>GSMSVQSGSTANLPADLATALATAKENDGHDFEAPKVGEDQGSPEVTDGPKTEEELLALEKEKPAEEKPKEDKPAAAKPETPKTVTPEWQTVEKKEQQGTVTIREEKGVRYNQLSSTAQNDNAGKPALFEKKGLTVDANGNATVDLTFKDDSEKGKSRFGVFLKFKDTKNNVFVGYDKDGWFWEYKSPTTSTWYRGSRVAAPETGSTNRLSITLKSDGQLNASNNDVNLFDTVTLP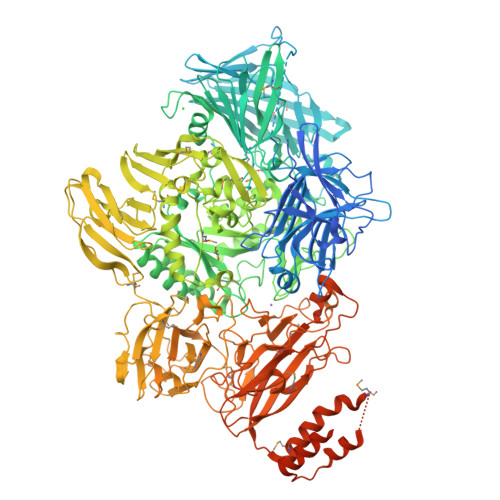AAVNDHLKNEKKILLKAGSYDDERTVVSVKTDNQEGVKTEDTPAEKETGPEVDDSKVTYDTIQSKVLKAVIDQAFPRVKEYSLNGHTLPGQVQQFNQVFINNHRITPEVTYKKINETTAEYLMKLRDDAHLINAEMTVRLQVVDNQLHFDVTKIVNHNQVTPGQKIDDERKLLSSISFLGNALVSVSSDQTGAKFDGATMSNNTHVSGDDHIDVTNPMKDLAKGYMYGFVSTDKLAAGVWSNSQNSYGGGSNDWTRLTAYKETVGNANYVGIHSSEWQWEKAYKGIVFPEYTKELPSAKVVITEDANADKKVDWQDGAIAYRSIMNNPQGWKKVKDITAYRIAMNFGSQAQNPFLMTLDGIKKINLHTDGLGQGVLLKGYGSEGHDSGHLNYADIGKRIGGVEDFKTLIEKAKKYGAHLGIHVNASETYPESKYFNEKILRKNPDGSYSYGWNWLDQGINIDAAYDLAHGRLARWEDLKKKLGDGLDFIYVDVWGNGQSGDNGAWATHVLAKEINKQGWRFAIEWGHGGEYDSTFHHWAADLTYGGYTNKGINSAITRFIRNHQKDAWVGDYRSYGGAANYPLLGGYSMKDFEGWQGRSDYNGYVTNLFAHDVMTKYFQHFTVSKWENGTPVTMTDNGSTYKWTPEMRVELVDADNNKVVVTRKSNDVNSPQYRERTVTLNGRVIQDGSAYLTPWNWDANGKKLSTDKEKMYYFNTQAGATTWTLPSDWAKSKVYLYKLTDQGKTEEQELTVKDGKITLDLLANQPYVLYRSKQTNPEMSWSEGMHIYDQGFNSGTLKHWTISGDASKAEIVKSQGANDMLRIQGNKEKVSLTQKLTGLKPNTKYAVYVGVDNRSNAKASITVNTGEKEVTTYTNKSLALNYVKAYAHNTRRNNATVDDTSYFQNMYAFFTTGSDVSNVTLTLSREAGDEATYFDEIRTFENNSSMYGDKHDTGKGTFKQDFENVAQGIFPFVVGGVEGVEDNRTHLSEKHDPYTQRGWNGKKVDDVIEGNWSLKTNGLVSRRNLVYQTIPQNFRFEAGKTYRVTFEYEAGSDNTYAFVVGKGEFQSGRRGTQASNLEMHELPNTWTDSKKAKKATFLVTGAETGDTWVGIYSTGNASNTRGDSGGNANFRGYNDFMMDNLQIEEITLTGKMLTENALKNYLPTVAMTNYTKESMDALKEAVFNLSQADDDISVEEARAEIAKIEALKNALVQKKTALVADDFASLTAPAQAQEGLANAFDGNLSSLWHTSWGGGDVGKPATMVLKEATEITGLRYVPRGSGSNGNLRDVKLVVT[2x]>GSHMASMSKIRVLCVDDSALMRQIMTEIINSHPDMEVVATAPDPLVARDLIKKFNPQVLTLDVEMPRMDGLDFLEKLMRLRPMPVVMVSSLTGKGSEITLRALELGAIDFVTKPQLGIREGMLAYSELIAEKIRMAAKARLPQRSTTAEPTKIIQHMPLLSSEKLIAIGASTGGTEAIRHVLQPLPPTSPALLITQHMPPGFTKSFAERLNKLCQITVKEAEDGERVLPGHAYIAPGARHLELARSGANYQVRLNDGPPVNRHRPSVDVLFRSVAQYAGRNAVGVILTGMGNDGAAGM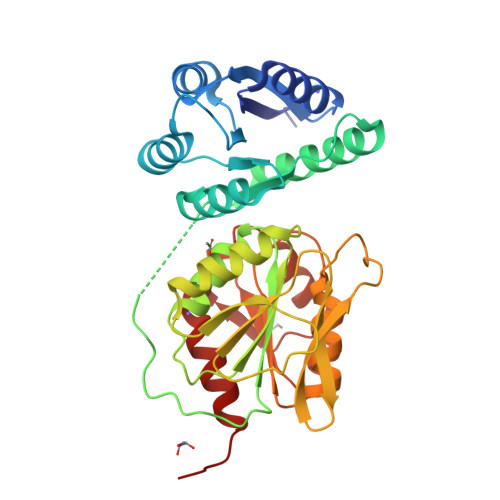LELHQAGAYTLAQNEASCVVFGMPREAIAMGGVDEVVDLHQVSQRMLAQISAGQALRI[5x]>[2x]LGSVKPATCEKPKFLEYKTCVGDLAVVIAKALDEFKEFCIVNAANEHMSHGGGVAKA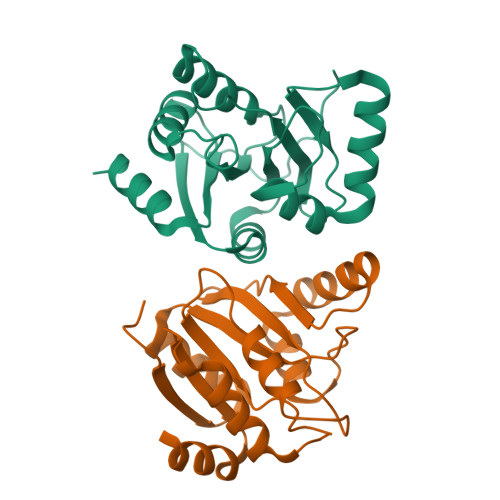IADFCGPDFVEYCADYVKKHGPQQKLVTPSFVKGIQCVNNVVGPRHGDSNLREKLVAAYKSVLVGGVVNYVVPVLSSGIFGVDFKISIDAMREAFKGCAIRVLLFSLSQEHIDYFDATCK The 22nd genetically encoded amino acid, pyrrolysine, plays a unique role in the key step in the growth of methanogens on mono-, di-, and tri-methylamines by activating the methyl group of these substrates for transfer to a corrinoid cofactor. A substrate:corrinoid methyltransferase catalyzes the demethylation of the specific methylamine, and subsequently transfers this methyl group onto an associated corrinoid protein. In summary, we have determined the structures of native MttB, and its complexes with a substrate analog, sulfite, and its physiological relevant corrinoid protein, MttC. These structures have provided new insights into the mechanism of activation of pyrrolysine that is distinct from the previously determined MtmB structure, and details of the key steps in the pyrrolysine-mediated transfer of methyl groups from methylamine substrates to the cobalamin cobalt in corrinoid proteins.

The 2.5 Å structure of MttB reveals that the protein exists as a D3-symmetric homo-hexamer, although based on the strong protein contacts between pairs of twofold related subunits, the structure is perhaps better considered a trimer-of-dimers. A C-terminal loop (residues 396–452) that directly follows the TIM-barrel domain in the sequence forms extensive contacts with a twofold related MttB subunit leading to formation of tightly associated MttB dimers. The dimer is further stabilized by interactions provided by an N-terminal β-strand (β2, residues 17–19). The major interaction is provided by an N-terminal α/β subdomain (residues 23–81) which lies near the threefold axis and is positioned on the opposite side of the TIM barrel relative to the dimerization loop. An α-helix (α3, residues 71–80) from this α/β subdomain interacts with the threefold related α helices on the other two dimers forming a triangle. A lone water appears to hydrogen bond the pyrroline imine and this water is in-turn stabilized by hydrogen bonding interactions with the hydroxyl group of Tyr364 and the main chain carbonyl of Gly110. Notably, the orientation of the Gly110 carbonyl is achieved by its participation in a Gly110-Thr111 cis peptide-bond. Based on the MttB structures, the mechanism of TMA addition to pyrrolysine to MttB appears to be much simpler than that of MtmB—involving only a single conformation of the pyrroline ring. One possibility is that Tyr364-Wat-Pyl334 form a proton shuttle that aids in the generation of the positively charged TMA-pyrrolysine adduct by formation of the tyrosine anion. It should be noted that the water that hydrogen bonds the pyrroline imine nitrogen in the native MttB structure is absent in both the sulfite-bond MttB and the MttB-MttC complex.

>MAKNNAVAGFNALNGVELNLFTTDELKAIHYATMEVLMDPGIQVSDPEARQIFKENGCEVNEKTNVVKIPEYLVRKALQLAPSRFVLWGRDKKFNTVQECGGKVHWTCFGTGVKVCKYQDGKYVTVDSVEKDIADIAKLCDWAENIDYFSLPVSARDIAGQGAQDVHETLTPLANTAKHFHHIDPVGENVEYYRDIVKAYYGGDEEEARKKPIFSMLLCPTSPLELSVNACQVIIKGARFGIPVNVLSMAMSGGSSPVYLAGTLVTHNAEVLSGIVLAQLTVPGAKVWYGSSTTTFDLKKGTAPVGSPELGLISAAVAKLAQFYGLPSYVAGSOSDAKVPDDQAGHEKTMTTLLPALAGANTIYGAGMLELGMTFSMEQLVIDNDIFSMVKKAMQGIPVSEETLAVESIQKVGIGNNFLALKQTRQLVDYPSNPMLLDRHMFGDWAAAGSKDLATVAHEKVEDVLKNHQVTPIDADIFKDMQAIVDKADKAFRGMGGHHHHHH[6x]> LCS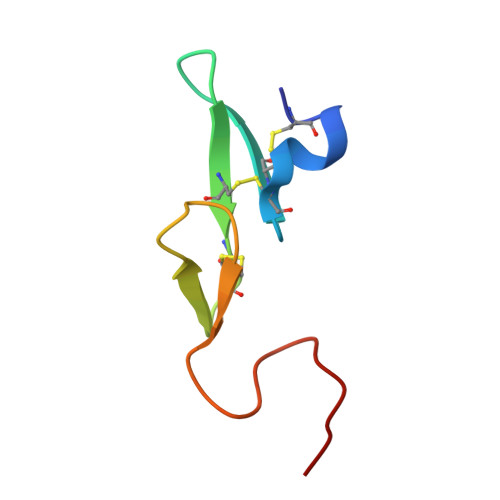LDNGDCDQFCHEEQNSVVCSCARGYTLADNGKACIPTGPYPCGKQTLE> DMFLYNLTLQRATGISFAIHGNFSGTKQQEIVVSRGKILELLRPDPNTGKVHTLLTVEVFGVIRSLMAFRLTGGTKDYIVVGSDSGRIVILEYQPSKNMFEKIHQETFGKSGCRRIVPGQFLAVDPKGRAVMISAIEKQKLVYILNRDAAARLTISSPLEAHKANTLVYHVVGVDVGFENPMFACLEMDYEEADNDPTGEAAANTQQTLTFYELDLGLNHVVRKYSEPLEEHGNFLITVPGGSDGPSGVLICSENYITYKNFGDQPDIRCPIPRRRNDLDDPERGMIFVCSATHKTKSMFFFLAQTEQGDIFKITLETDEDMVTEIRLKYFDTVPVAAAMCVLKTGFLFVASEFGNHYLYQIAHLGDDDEEPEFSSAMPLEEGDTFFFQPRPLKNLVLVDELDSLSPILFCQIADLANEDTPQLYVACGRGPRSSLRVLRHGLEVSEMAVSELPGNPNAVWTVRRHIEDEFDAYIIVSFVNATLVLSIGETVEEVTDSGFLGTTPTLSCSLLGDDALVQVYPDGIRHIRADKRVNEWKTPGKKTIVKCAVNQRQVVIALTGGELVYFEMDPSGQLNEYTERKEMSADVVCMSLANVPPGEQRSRFLAVGLVDNTVRIISLDPSDCLQPLSMQALPAQPESLCIVEMGGTEKQDELGERGSIGFLYLNIGLQNGVLLRTVLDPVTGDLSDTRTRYLGSRPVKLFRVRMQGQEAVLAMSSRSWLSYSYQSRFHLTPLSYETLEFASGFASEQCPEGIVAISTNTLRILALEKLGAVFNQVAFPLQYTPRKFVIHPESNNLIIIETDHNAYTEATKAQRKQQMAEEMVEAAGEDERELAAEMAAAFLNENLPESIFGAPKAGNGQWASVIRVMNPIQGNTLDLVQLEQNEAAFSVAVCRFSNTGEDWYVLVGVAKDLILNPRSVAGGFVYTYKLVNNGEKLEFLHKTPVEEVPAAIAPFQGRVLIGVGKLLRVYDLGKKKLLRKCENKHIANYISGIQTIGHRVIVSDVQESFIWVRYKRNENQLIIFADDTYPRWVTTASLLDYDTVAGADKFGNICVVRLPPNTNDEVDEDPTGNKALWDRGLLNGASQKAEVIMNYHVGETVLSLQKTTLIPGGSESLVYTTLSGGIGILVPFTSHEDHDFFQHVEMHLRSEHPPLCGRDHLSFRSYYFPVKNVIDGDLCEQFNSMEPNKQKNVSEELDRTPPEVSKKLEDIRTRY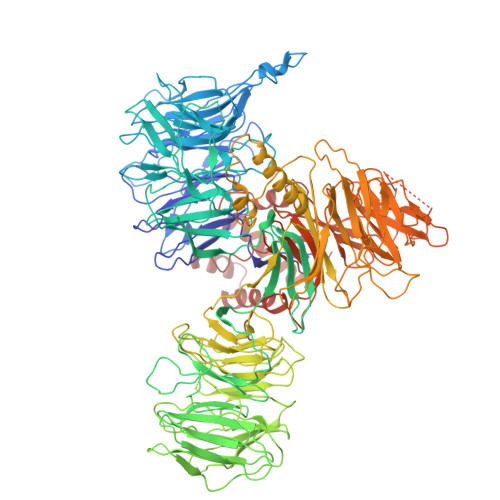AFDYKDD>[4x]LPSPTPNLEIKYTKIFINNEWQNSESGRVFPVYNPATGEQVCEVQEADKADIDKAVQAARLAFSLGSVWRRMDASERGRLLDKLADLVERDRAVLATMESLNGGKPFLQAFYVDLQGVIKTFRYYAGWADKIHGMTIPVDGDYFTFTRHEPIGVCGQIIPWNFPLLMFAWKIA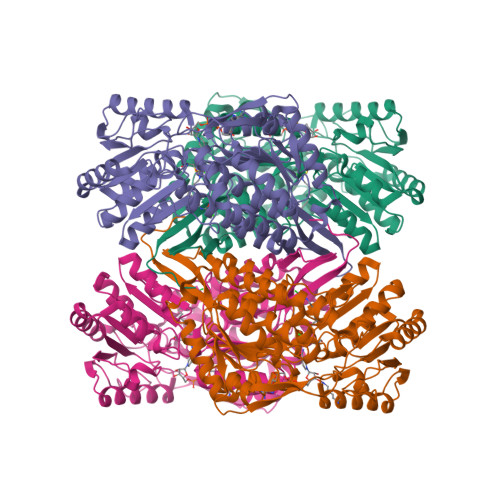PALCCGNTVVIKPAEQTPLSALYMGALIKEAGFPPGVINILPGYGPTAGAAIASHIGIDKIAFTGSTEVGKLIQEAAGRSNLKRVTLELGGKSPNIIFADADLDYAVEQAHQGVFFNQGQCCTAGSRIFVEESIYEEFVRRSVERAKRRVVGSPFDPTTEQGPQIDKKQYNKILELIQSGVAEGAKLECGGKGLGRKGFFIEPTVFSNVTDDMRIAKEEIFGPVQEILRFKTMDEVIERANNSDFGLVAAVFTNDINKALTVSSAMQAGTVWINCYNALNAQSPFGGFKMSGNGREMGEFGLREYSEVKTVTVKIPQKNS> MSKQFVRSAKNMMKGYSSTQVLVRDATANDSRTPSIDTLDDLAQRSYDSVDFFEIMDMLDKRLNDKGKYWRHVAKSLTVLDYLVRFGSENCVLWCRENFYVIKTLREFRHENESGFDEGQIIRVKAKELVSLLNDEER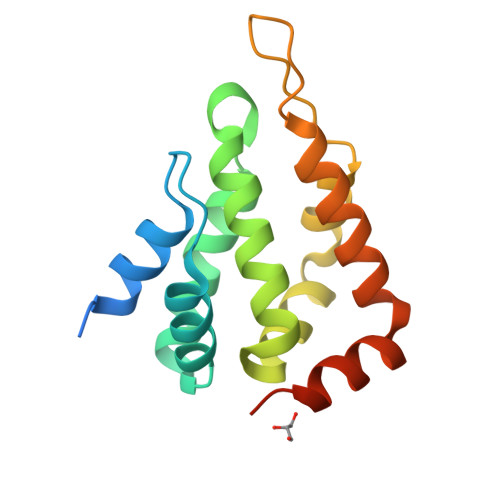LREERSMNTRNRRANRAA> GLGDELEEVIVEKTKQTVASISSGPKHTQKVPILTANETGATMPVLPSDSIETRTTYMHFNGSETDVECFLGRAACVHVTEIQNKDATGIDNHREAKLFNDWKINLSSLVQLRKKLELFTYVRFDSEYTILATASQPDSANYSSNLVVQAMYVPPGAPNPKEWDDYTWQSASNPSVFFKVGDTSRFSLPYVGLASAYNCFYDGYSHDDAETQYGITVLNH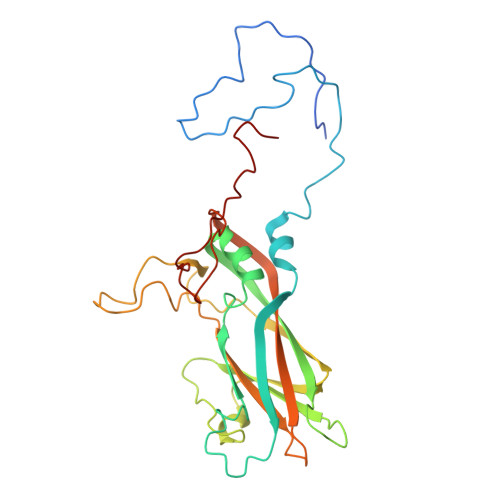MGSMAFRIVNEHDEHKTLVKIRVYHRAKHVEAWIPRAPRALPYTSIGRTNYPKNTEPVIKKRKGDIKSY> AGFGAQHRKMGKSLYLRNEVFAAWIEKVDALVQDELGYSVLELILDDAQDYGIETTQVTIFAIQI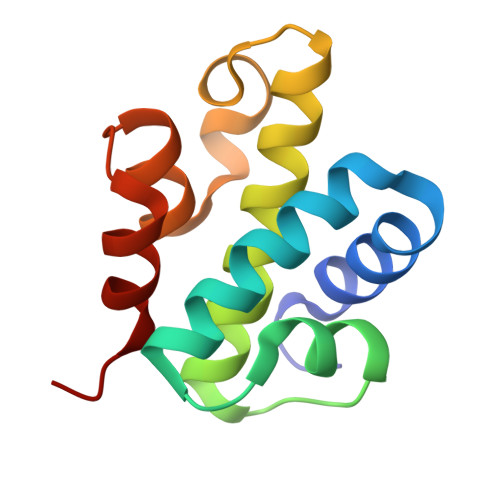ALGELLRHHGAKPAAVIGQSLGEAASAYFAGGLSLRDATRAICSRS> VIVTRSGAILPKPVKMSFG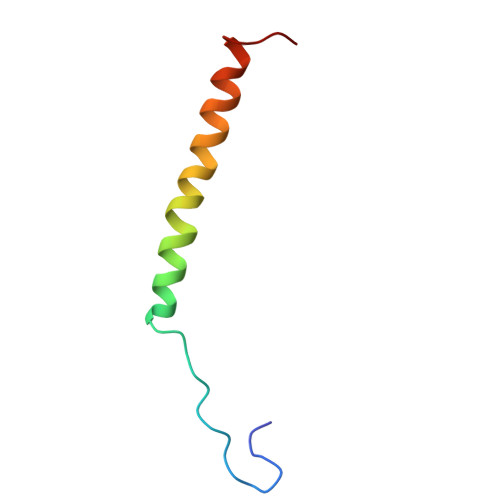LLRVFSIVIPFLYVGTLISKNFAALLEEHDIF>[2x]SMAEIKQGIREVILCKDQDGKIGLRLKSIDNGIFVQLVQANS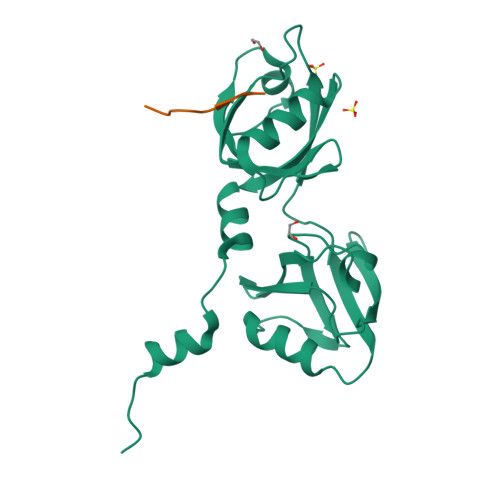PASLVGLRFGDQVLQINGENCAGWSSDKAHKVLKQAFGEKITMTIRDRPFERTITMHKDSTGHVGFIFKNGKITSIVKDSSAARNGLLTEHNICEINGQNVIGLKDSQIADILSTSGTVVTITIMPAFIFEHIIKRMAPSIMKSLMDHTIPEV;>[2x]APTNEFYA>[12x]GHMSEEQVAQDTEEVFRSYVFYRHQQEQEAEGVAAPAD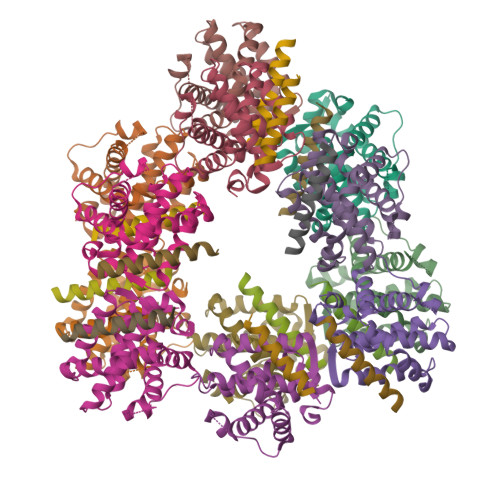PEMVTLPLQPSSTMGQVGRQLAIIGDDINRRYDSEFQTMLQHLQPTAENAYEYFTKIATSLFESGINWGRVVALLGFGYRLALHVYQHGLTGFLGQVTRFVVDFMLHHSIARWIAQRGGWVAALNLGN;>GHMEEIIHKLAMQLRHIGDNIDHRMVRED[12x]> AEDCGIPESIENGKVEDPESTLFGSVIRYTCEEPYYYMENGGGGEYHCAGNGSWVNEVLGPELPKCVPVCGVPREPFEEKQRIIGGSDADIKNFPWQVFFDNPWAGGALINEYWVLTAAHVVEGNREPTMYVGSTSVQTSRLAKSKMLTPEHVFIHPGWKLLEVPEGRTNFDNDIALVRLKDPVKMGPTVSPICLPGTSSDYNLMDGDLGLISGWGRTEKRDRAVRLKAARLPVAPLRKCKE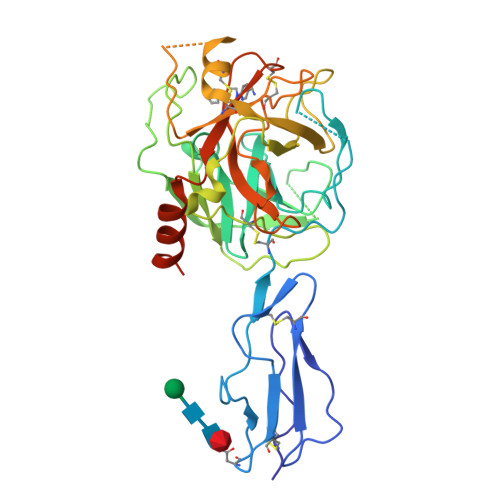VKVEKPTADAEAYVFTPNMICAGGEKGMDSCKGDSGGAFAVQDPNDKTKFYAAGLVSWGPQCGTYGLYTRVKNYVDWIMKTMQENSTPREDGSGHHHHHHHH> VTEGPYKLPPGWRWVRLGEVCLPTER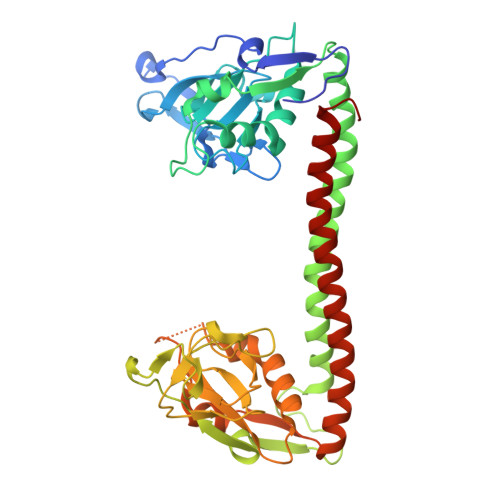RDPTKNPSTYFVYVDISAIDSTVGKIVSPKEILGQHAPSRARKVIRSGDVIFATTRPYLKNIALVPPDLDGQICSTGFCVIRANREFAEPEFLFHLCRSDFITNQLTASKMRGTSYPAVTDNDVYNTLIPLPPLEEQRRIVAKVEALMERVREVRRLRAEAQKDTELLMQTALAEVFPHPGADLPPGWRWVRLGEVCDIIMGQSPPSSTYNFEGNGLPFFQGKADFGDLHPTPRIWCSAPQKVARPGDVLISVRAPVGSTNVANLACCIGRGLAALRPRDSLERFWLLYYLHYLEPELSKMGAGSTFNAITKKDLQNVFIPLPPLEEQRRIVAYLDQIQQQVAALKRAQAETEAELKRLEQAILDKAFRGDL> 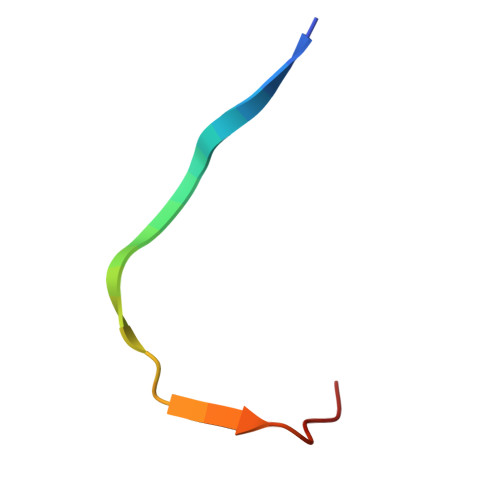MLRTMLKSKIHRATVTCADLHYVG> MRGSHHHHHHENLYFQGSLAVAEPVVNAADAKGTNVNDKVTASDFKLEKTAFDPNQSGNTFMAANFKVTGQVKSGDYFTAKLPDSVTGNGDVDYSNSNNTMPIADIKSTNGDVVAKATYDILTKTYTFVFTDYVNDKENINGQFSLPLFTDRAKAPKSGTYDANINIADEMFDNKITYNYSSPIAGIDKPNGANISSQIIGVDTASGQNTYKQTVFVNPKQRVLGNTWVYIKGYQDKIEESSGKVSATDTKLRIFEVNDTSKLSDSYYADPNDSNLKEVTGEFKDKISYKYDNVASINFGDINKTY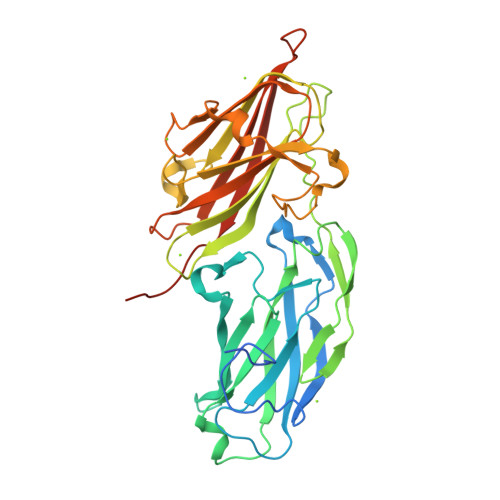VVLVEGHYDNTGKNLKTQVIQENIDPATGKDYSIFGWNNENVVRYGGGSADGDSAVN> GLGQMLESMIDNTVRETVGAATSRDALPNTEASGPTHSKEIPALTAVETGATNPLVPSDTVQTRHVVQHRSRSESSIESFFARGACVTIMTVDNSASTTNKDKLFAVWKITYKDTVQLRRKLEFFTYSRFDMELTFVVTANFTETNNGHALNQVYQIMYVPPGAPVPEKWDDYTWQTSSNPSIFYTYGTAPARISVP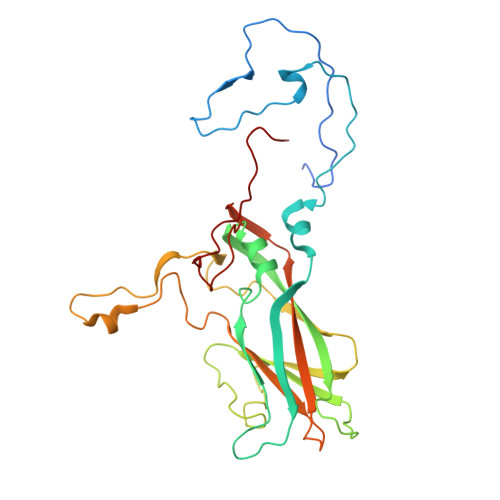YVGISNAYSHFYDGFSKVPLKDQSAALGDSLYGAASLNDFGILAVRVVNDHNPTKVTSKIRVYLKPKHIRVWCPRPPRAVAYYGPGVDYKDGTLTPLSTKDLTTY> MELIQDTSRPPLEYVKGVPLIKYFAEALGPLQSFQARPDDLLISTYPKSGTTWVSQILDMIYQGGDLEKCHRAPIFMRVPFLEFKAPGIPSGMETLKDTPAPRLLKTHLPLALLPQTLLDQKVKVVYVARNAKDVAVSYYHFYHMAKVHPEPGTWDSFLEKFMVGEVSYGSWYQHVQEWWELSRTHPVLYLFYEDMKENPKREIQKILEFVGRSLPEETVDFVVQHTS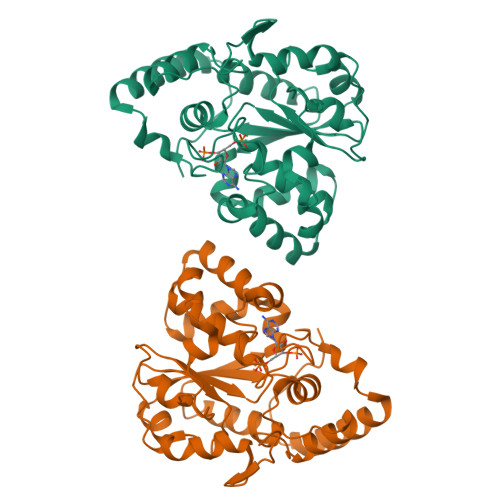FKEMKKNPMTNYTTVPQEFMDHSISPFMRKGMAGDWKTTFTVAQNERFDADYAEKMAGCSLSFRSEL> MAAIGRGRSLKNLRVRGRNDSGEENVPLDLTREPSDNLREILQNVARLQGVSNMRKLGHLNNFTKLLCDIGHSEEKLGFHYEDIIICLRLALLNEAKEVRAAGLRALRYLIQDSSILQKVLKLKVDYLIARCIDIQQSNEVERTQALRLVRKMITVNASLFPSSVTNSLIAVGNDGLQERDRMVRACIAIICELALQNPEVVALRGGLNTILKNVIDCQLSRINEALITTILHLLNHPKTRQYVRADVELERILAPYTDFHYRHSPDTAEGQLKEDREARFLASKMGIIATFRSWAGIINLCKPGNSGIQSLIGVLCIPNMEIRRGLLEVLYDIFRLPLPVVTEEFIEALLSVDPGRFQDSWRLSDGFVAAEAKTILPHRARSRPDLMDNYLALILSAFIRNGLLEGLVEVITNSDDHISVRATILLGELLHMANTILPHSHSHHLHCLPTLMNMAASFDIPKEKRLRASAALNCLKRFHEMKKRGPKPYSLHLDHIIQKAIATHQKRDQYLRVQKDIFILKDTEEALLINLRDSQVLQHKENLEWNWNLIGTILKWPNVNLRNYKDEQLHRFVRRLLYFYKPSSKLYANLDLDFAKAKQLTVVGCQFTEFLLESEEDGQGYLEDLVKDIVQWLNASSGMKPERSLQNNGLLTTLSQHYFLFIGTLSCHPHGVKMLEKCSVFQCLLNLCSLKNQDHLLKLTVSSLDYSRDGLARVILSKILTAATDACRLYATKHLRVLLRANVEFFNNWGIELLVTQLHDKNKTISSEALDILDEACEDKANLHALIQMKPALSHLGDKGLLLLLRFLSIPKGFSYLNERGYVAKQLEKWHREYNSKYVDLIEEQLNEALTTYRKPVDGDNYVRRSNQRLQRPHVYLPIHLYGQLVHHKTGCHLLEVQNIITELCRNVRTPDLDKWEEIKKLKASLWALGNIGSSNWGLNLLQEENVIPDILKLAKQCEVLSIRGTCVYVLGLIAKTKQGCDILKCHNWDAVRHSRKHLWPVVPDDVEQLCNELSSIPSTLSLNSESTSSRHNSESESVPSSMFILEDDRFGSSSTSTFFLDINEDTEPTFYDRSGPIKDKNSFPFFASSKLVKNRILNSLTLPNKKHRSSSDPKGGKLSSESKTSNRRIRTLTEPSVDFNHSDDFTPISTVQKTLQLETSFMGNKHIEDTGSTPSIGENDLKFTKNFGTENHRENTSRERLVVESSTSSHMKIRSQSFNTDTTTSGISSMSSSPSRETVGVDATTMDTDCGSMSTVVSTKTIKTSHYLTPQSNHLSLSKSNSVSLVPPGSSHTL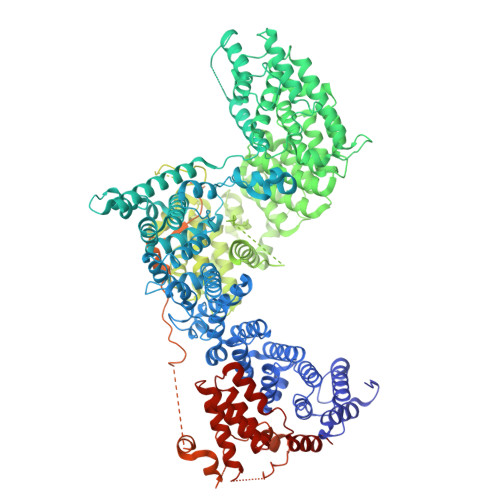PRRAQSLKAPSIATIKSLADCNFSYTSSRDAFGYATLKRLQQQRMHPSLSHSEALASPAKDVLFTDTITMKANSFESRLTPSRFMKALSYASLDKEDLLSPINQNTLQRSSSVRSMVSSATYGGSDDYIGLALPVDINDIFQVKDIPYFQTKNIPPHDDRGARAFAHDAGGLPSGTGGLVKNSFHLLRQQMSLTEIMNSIHSDASLFLESTEDTGLQEHTDDNCLYCVCIEILGFQPSNQLSAICSHSDFQDIPYSDWCEQTIHNPLEVVPSKFSGISGCSDGVSQEGSASSTKSTELLLGVKTIPDDTPMCRILLRKEVLRLVINLSSSVSTKCHETGLLTIKEKYPQTFDDICLYSEVSHLLSHCTFRLPCRRFIQELFQDVQFLQMHEEAEAVLATPPKQPIVDTSAES>MSQTNANDLRNNEVFFISPSNNTNKVLDKISQSEVKLWNKLSGANQKWRLIYDTNKQAYKIKVMDNTSL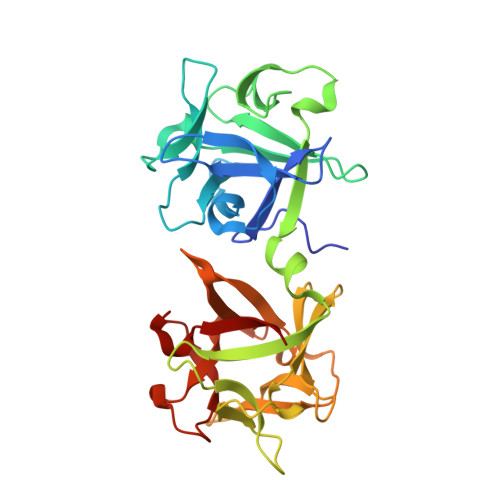ILTWNAPLSSVSVKTDTNGDNQYWYLLQNYISRNVIIRNYMNPNLVLQYNIDDTLMVSTQTSSSNQFFKFSNCIYEALNNRNCKLQTQLNSDRFLSKNLNSQIIVLWQWIDSSRQKWIIEYNETKSAYTLKCQENNRYLTWIQNSNNYVETYQSTDSLIQYWNINYLDNDASKYILYNLQDTNRVLDVYNSQIANGTHVIVDSYHGNTNQQWIINLI[2x]>[2x]HMMGGISICVATDCDGEKVNLRFLFDAAGPSVSRLLNYSTTAFNNYFRLKGISRAFAVNSAVVFNDVHCTWDRLERTTQLLHNSQVYLFQPDTLDIPAAIPEPYEGEPLLSA;>SSLSPY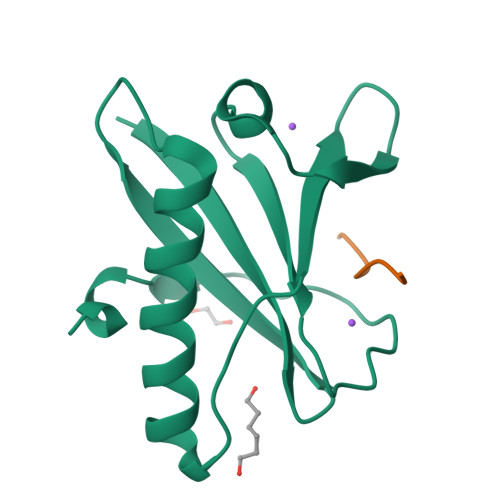LRYLPSDVSGGEWDKPDVGDVLCFQAKEPQRRRVLTSPVPDELLIK[2x]>[2x]MKMIVGLGNPGTKYQYTKNNIGFMVVDKIAREHQATFKKNPFEAEVAEFFHNGEKILLVKP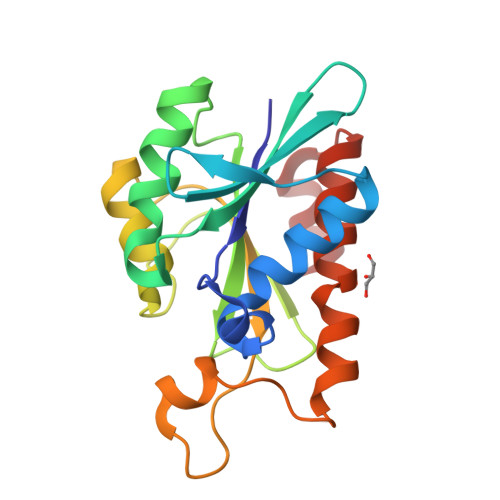QTFMNESGRAVGPLMTYFGIYPEELVVIYDDLDLAVGKIRLRQKGSAGGHNGIKSIISHLNTNVFDRIKVGIGRPEGKKTVVQHVLSPFSKENQPLIEESMCQSVKAVEYLIEGHSFVDAMNRFN>GAMAKTTNAGKRNMAPTLPNPLRNELVSKQKLAELSSIIDGEFEPIQRKAPSPRGRLGRRVKLRKHLVEINADEITITLSRYTSPEALERSITALAAMTGHAPSSIKEECVELIDKLDWLRVENDVIQYPTLSKLLELYNSQNESKHLSIEKLIAGLAVRRKVCKLVQDGHIDETVYRALDEMAAGA[2x]

The replication of the two chromosomes in the pathogenic bacterium Vibrio cholerae is coordinated by the binding of initiator protein RctB to a checkpoint sequence, crtS. V. cholerae Chr2 originates from an iteron-type plasmid, evident from its replication origin (ori2) and initiator (RctB). RctB is divided into four structural regions (I–IV)14. Domains, I, II and III, interact with DNA via Helix-Turn-Helix (HTH) motifs and are essential for ori2 replication.

The C-terminal domain (IV) is essential for down-regulating Chr2 initiation and has been shown in vitro to play a crucial role in self-interaction, promoting cooperative DNA binding and oligomerization. The C-terminal region of RctB, named domain IV (RctBIV), is critical to downregulate Chr2 copy number through its involvement, directly or indirectly, in handcuffing activities and binding to 29/39 m15,16,29. The structure of RctBIV reveals that it is organized into two structural subdomains connected by an extended linker or hinge region. The N-terminal subdomain consists of a 3-stranded β-sheet stacking two α-helices and the C-terminal subdomain has 4 α-helices in a bundle. In the crystal, RctBIV retains a dimeric association, confirmed by Size Exclusion Chromatography (SEC). This dimerization is primarily mediated by a β-sheet (β3) spanning residue 545 to 549 and involves an interface of 392.4 Å2 (primary interface). The crystal lattice contacts of the C-terminal subdomain suggest the presence of a secondary interaction interface involving 315.4 Å2, which could mediate further oligomerization via this region (secondary interface). A DALI31 search confirmed the C-terminal subdomain as a protein recognition domain capable of forming transient homodimeric interfaces, with Z-scores between 3.7 and 5.4. Thus, RctBIV can form homodimers via two different regions: at a primary interface formed between the β3 sheets and at the secondary interface between α-helices. Collectively these results suggest that RctBIV could be an anchor not only for dimerization but also for the formation of transient oligomeric structures when bound to DNA or even to bridge two chromosomal regions.> SMRIGANGDETVWADEEFAGRDFRDEDLSRIRTERVVFTECD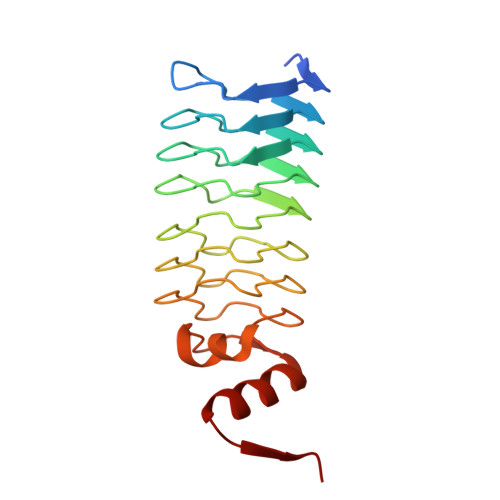FSGVDLSESEHHGSAFRNCTFRRSTIWHSTFTNCSLLGSVFTECRIRPVTFVECDFTLAVLGGCDLRAVDLSDCRLREVSLVGADLRKAVLRRADLTGSRVQDARLEEADLRGTRVDPTFWTTAKVRGAKIDIEQALAYAAAHGLAVHGG Here, we have determined the structure and molecular architecture of the Ty3 capsid by 3D and 2D cryo-electron microscopy (cryo-EM) and compared it with those of the retroviruses. In the case of Ty3, Gag3 is cleaved into CA and NC domains. Formation of the capsid is important for genome protection and is an essential step in the retroelement life cycle. Similar to retroviruses, the protruding capsomers of the Ty3 capsid are formed by the CA-NTD, while the inner layer, linking the capsomers together, is formed by the CA-CTD.

Adjacent CA-NTD domains exist in different orientations; therefore, we considered a pair of CA-NTDs [one in orientation A (cyan) and one in orientation B (dark blue)] to be the repeating unit, and aligned and averaged the four independent copies of this pair of CA-NTDs (excluding the CA-NTDs from the fivefold position). In this way, we generated a higher resolution 5.5-Å map of the CA-NTDs. We flexibly fit the homology model of the Ty3 CA-NTD into the new EM map. The N-terminal 36 amino acids of the CA-NTD do not have a defined secondary structure in the homology model; however, in our map, we resolve density corresponding to this region. This density runs outwards along the interface between helix 1 and helix 2 of the CA-NTD in the middle of the threefold (and fivefold) position for ∼60 Å (cyan and blue densities). Interactions between these N-terminal parts of CA-NTDs may contribute to stabilization of the structure at threefold and fivefold positions (central densities). In orientation B, this density continues over the top of the CA-NTD and down the interface of helix 3 of one CA-NTD and helix 1 of the neighboring CA-NTD on the outer side of the threefold position (blue density). The total length of the density in orientation B in the EM map is ∼100 Å and likely accommodates all 36 amino acids. In conformation A, the N-terminal half of the density is not visible; it is not bound to the rest of the CA-NTD and is probably disordered. Instead, the surface of CA-NTD helix 3, where it would otherwise be bound, is occluded by binding the neighboring CA-NTD.

>MSFMDQIPGGGNYPKLPVECLPNFPIQPSLTFRGRNDSHKLKNFISEIMLNMSMISWPNDASRIVYCRRHLLNPAAQWANDFVQEQGILEITFDTFIQGLYQHFYKPPDINKIFNAITQLSEAKLGIERLNQRFRKIWDRMPPDFMTEKAAIMTYTRLLTKETYNIVRMHKPETLKDAMEEAYQTTALTERFFPGFELDADGDTIIGATTHLQEEYDSDYDSEDNLTQNRYVHTVRTRRSYNKPMSNHRNRRNNNASREECIKNRLCFYCKKEGHRLNECRARKAVLTDLELESKDQQTLFIKTLPIVH[2x]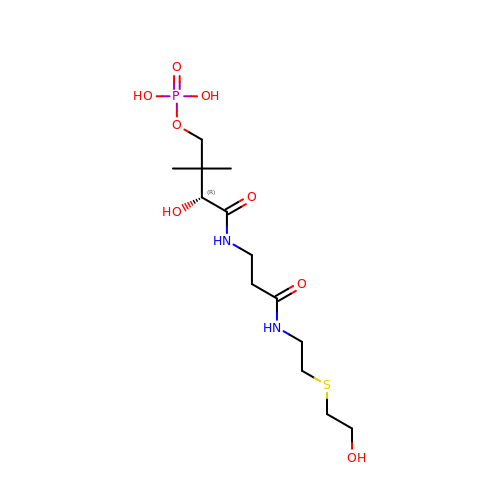N~3~-[(2R)-2-hydroxy-3,3-dimethyl-4-(phosphonooxy)butanoyl]-N-{2-[(2-hydroxyethyl)sulfanyl]ethyl}-beta-alaninamide | C13 H27 N2 O8 P S | IGYAFBQHDWNTQK-NSHDSACASA-N> MIAPLILYLDVPFTTFRESHAREMGKTYPVPPPATVYGMLLSLVGETNVYRHCGVELAIAMLSSPKKSRILRQMRRFKNADFSHPENVIPCYQEILSNLKCLIWVRSDEEKIQPSLRERIQLAFDHPELVRRFGCLFLGESDQLIKTI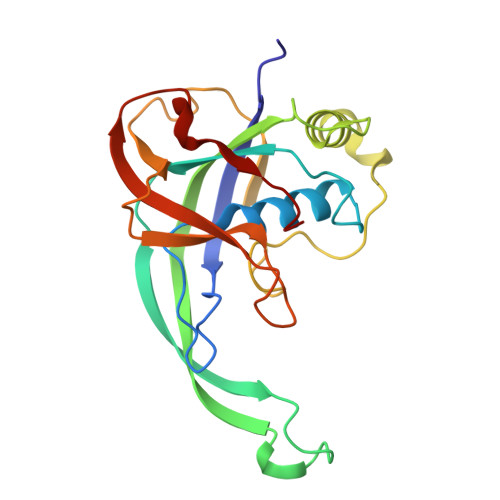KLAREDYLEGVRQWAIRDNRGRLTLPYWVDHVGSRNTRFLRYRIEEMDRLSPPDLAWTMVQSPI>[6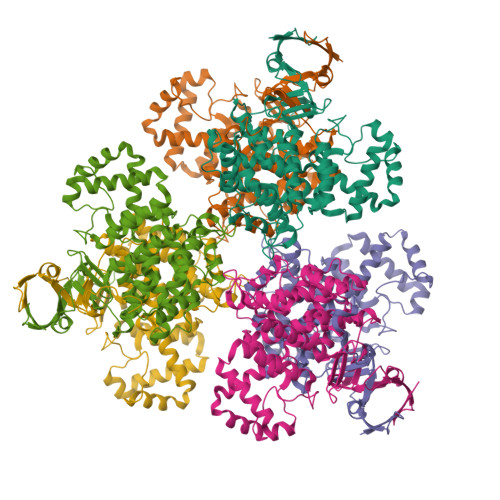x]MADKKAQLIIEGSAPVELPVLSGTMGPDVVDVRGLTATGHFTFDPGFMSTASCESKITYIDGDKGVLLHRGYPIEQLAEKSDYLETCYLLLNGELPTAAQKEQFVGTIKNHTMVHEQLKTFFNGFRRDAHPMAVMCGVIGALSAFYHDSLDINNPKHREVSAHRLIAKMPTIAAMVYKYSKGEPMMYPRNDLNYAENFLHMMFNTPCETKPISPVLAKAMDRIFILHADHEQNASTSTVRLAGSSGANPFACIASGIAALWGPAHGGANEAVLRMLDEIGDVSNIDKFVEKAKDKNDPFKLMGFGHRVYKNFDPRAKVMKQTCDEVLQELGINDPQLELAMKLEEIARHDPYFVERNLYPNVDFYSGIILKAIGIPTSMFTVIFALARTVGWISHWQEMLSGPYKIGRPRQLYTGHTQRDFTALKDRG>[4x]HMDKLPNIVILATGGTIAGSAATGTQTTGYKIGALGVDTLINAVPEVKKLANVKGEQFSNMASQNMTGDVVLKLSQRVNELLARDDVDGVVITHGTDTVEESAYFLHLTVKSDKPVVFVAAMRPATAISADGPMNLLEAVRVAGDKQSRGRGVMVVLNDRIGSARYITKTNASTLDTFKANEEGYLGVIIGNRIYYQNRIDKLHTTRSVFDVR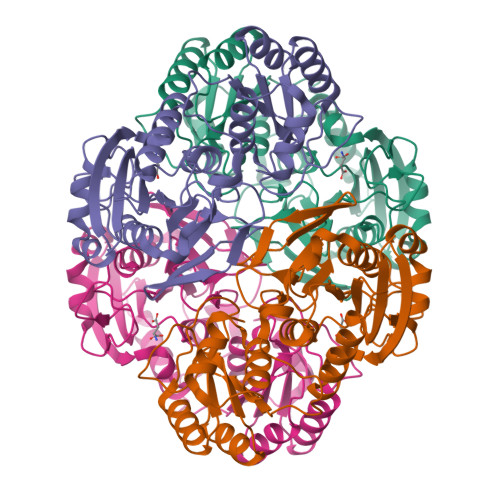GLTSLPKVDILYGYQDDPEYLYDAAIQHGVKGIVYAGMGAGSVSVRGIAGMRKAMEKGVVVIRSTRTGNGIVPPDEELPGLVSDSLNPAHARILLMLALTRTSDPKVIQEYFHTY>MPEGPELHLASQFVNEACRALVFGGCVEKSSVSRNPEVPFESSAYRISASARGKELRLILSPLPGAQPQQEPLALVFRFGMSGSFQLVPREELPRHAHLRFYTAPPGPRLALCFVDIRRFGRWDLGGKWQPGRGPCVLQEYQQFRENVLRNLADKAFDRPICEALLDQRFFNGIGNYLRAEILYRLKIPPFEKARSVLEALQQHRPSPELTLSQKIRTKLQNPDLLELCHSVPKEVVQLGGRGYGSESGEEDFAAFRAWLRCYGMPGMSSLQDRHGRTIWFQGDPGPLAPKGRKSRKKKSKATQLSPEDRVEDALPPSKAPSRTRRAKRDLPKRTATQ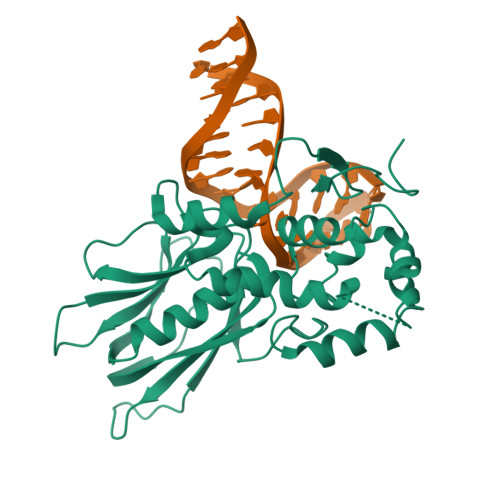RPEGTSLQQDPEAPTVPKKGRRKGRQAASGHCRPRKVKADIPSLEPEGTSASAALGHHHHHH[3x]> QDSTSDLIPAPPLSKVPLQQNFQDNQFHGKWYQVGRAGNAAPPMDPELLLLTAQTYELKEDKSYDVTAVRFRKKMCEYLTMTFVPSPQPGEFTLGNIKNYPGLTSYFVRVVSTNYNQHAMVFFKKVQQNREYFSISLLGRTKELASELKENFIRFSKSLGLPENHIVFPVPIDQCIDGSA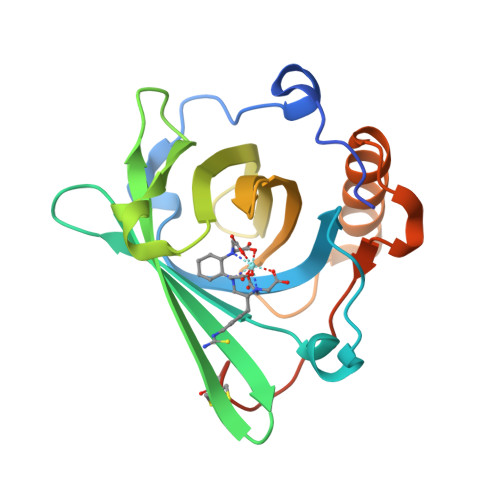WSHPQFEK> GSPKNYIEMKPHPWFFGKIPRAKAEEMLSKQRHDGAFLIRESESAPGDFSLSVKFGNDVQHFKVLRDGAGKYFLWVVKFNSLNELVDY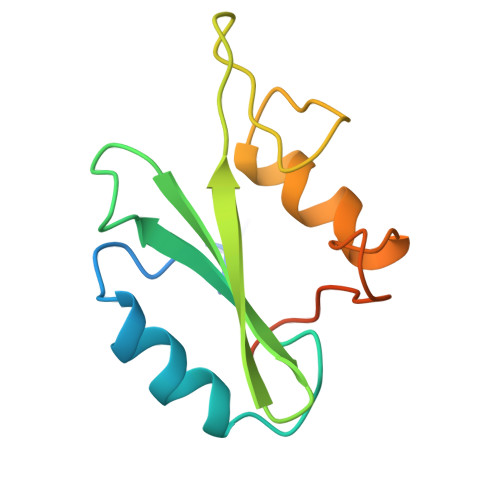HRSTSVSRNQQIFLRDIEQVPQQPTYVQA> MRRFCFPVATFAQAALRHRGIRWNTTMADNESHTGAKSSASSSTPSEANEISAMERASEARREIHDLWMSTEKMLDLENRVRSVASLIEKYKLDPSTPRENDVSRGLGDAFDRLLLLCVPLGKDSSKGTDDLERLMNLAGRNGREISVRTIQHLFARTDSFSEALAVFYAMRRCHVAMNMEAYYAMLYSLQRLEEEGWAQRFREECEEKGGVSEQAMDFVVKGINNALLPENKPWLGRVMFGDRDAPAQRREARDY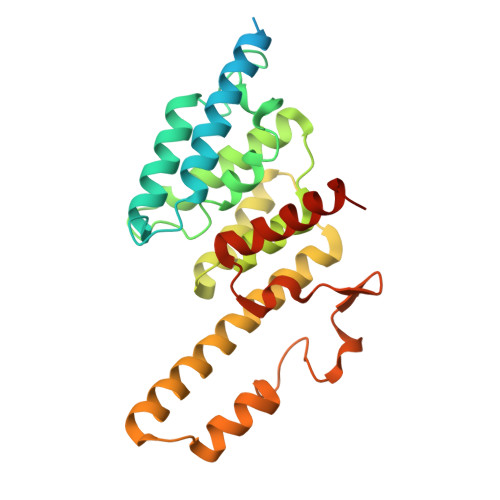DELSAMWTERYRDGSAFPTSP sclareol | C20 H36 O2 | 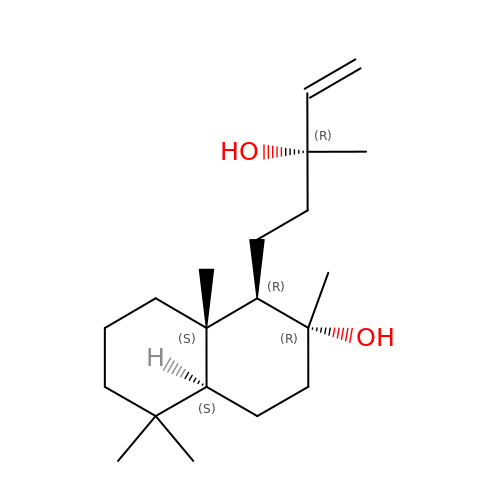XVULBTBTFGYVRC-HHUCQEJWSA-N(4~{S})-6-azanyl-3-methyl-4-[3-[4-(phenylmethyl)sulfonylphenyl]-5-(trifluoromethyl)phenyl]-4-propan-2-yl-2~{H}-pyrano[2,3-c]pyrazole-5-carbonitrile | C31 H27 F3 N4 O3 S | 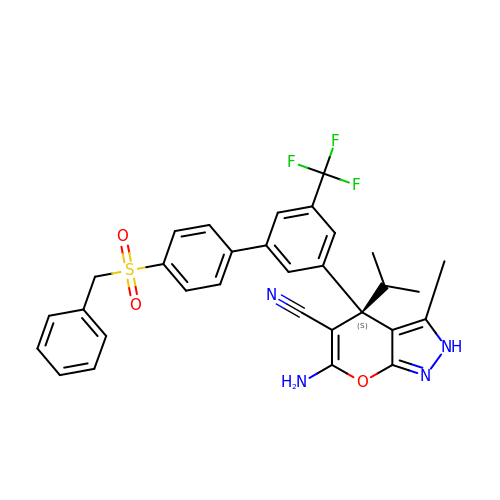PGTUNNBRJSLXTJ-PMERELPUSA-N>APQQINDIVHRTITPLIEQQKIPGMAVAVIYQGKPYYFTWGYADIAKKQPVTQQTLFELGSVSKTFTGVLGGDAIARGEIKLSDPTTKYWPELTAKQWNGITLLHLATYTAGGLPLQVPDEVKSSSDLLRFYQNWQPAWAPGTQRLYANSSIGLFGALAVKPSGLSFEQAMQTRVFQPLKLNHTWINVPPAEEKNYAWGYREGKAVHVSPGALDAEAYGVKSTIEDMARWVQSNLKPLDINEKTLQQGIQLAQSRYWQTGDMYQGLGWEMLDWPVNPDSIINGSDNKIALAARPVKAI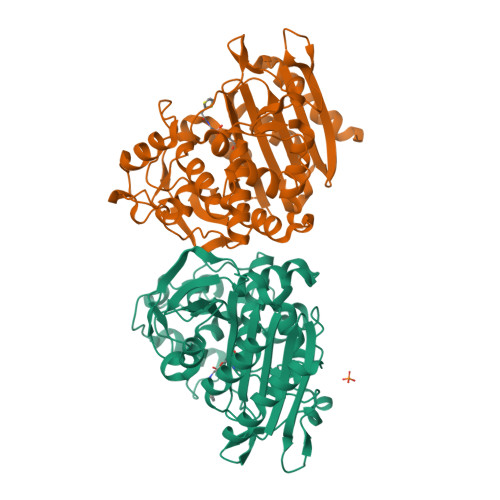TPPTPAVRASWVHKTGATGGFGSYVAFIPEKELGIVMLANKNYPNPARVDAAWQILNALA[2x]The final step of PG biosynthesis in Mtb is catalyzed by two different classes of enzymes, namely the D,D-transpeptidases (also known as Penicillin Binding Proteins – PBPs) and L,D-transpeptidases (Ldts). Conversely, Ldts catalyze the crosslinking of disaccharyl-tetrapeptide polymers by forming a transpeptide bond between the third amino acid in adjacent stem peptides thereby generating 3 → 3 crosslinkages between mDAP residues. Approximately two-thirds of the linkages in Mtb PG are of 3 → 3 type and their synthesis is catalyzed by the Ldts, highlighting the importance of these non-classical transpeptidases to this pathogen. Mtb lacking LdtMt2 is severely attenuated for growth, virulence, has deformed cell walls and exhibits an increased susceptibility to β-lactams.

apo and enzyme reacted with biapenem or tebipenem, and collected X-ray diffraction data at 2.49, 2.18 and 2.45 Å resolutions, respectively. All crystal forms belong to the monoclinic P21 space group with similar cell dimensions and contain two molecules per asymmetric unit. The apo and holo structures show negligible differences among them. The RMSDs are 0.4 and 0.3 Å between apo-LdtMt2 and LdtMt2-biapenem or LdtMt2-tebipenem, respectively, and 0.17 Å between the holo structures for the same 702 aligned Cα atoms aligned. Interestingly, the electron densities in these complexes are similar in size and shape. The observed densities are larger than the glycerol molecule observed in the apo-LdtMt2 crystal form but smaller than expected for an intact biapenem or tebipenem adduct as illustrated in Fig. 1d. The glycerol molecule found in the apo-LdtMt2 crystal form is disconnected at 2.7 Å from the catalytic cysteine and poorly overlapping with the larger and connected MTOA adduct.

>DLLVPKLTASVTDGAVGVTVDAPVSVTAADGVLAAVTMVNENGRPVAGRLSPDGLRWSTTEQLGYNRRYTLNATALGLGGAATRQLTFQTSSPAHLTMPYVMPGDGEVVGVGEPVAIRFDENIADRGAAEKAIKITTNPPVEGAFYWLNNREVRWRPEHFWKPGTAVDVAVNTYGVDLGEGMFGEDNVQTHFTIGDEVIATADDNTKILTVRVNGEVVKSMPTSMGKDSTPTANGIYIVGSRYKHIIMDSSTYGVPVNSPNGYRTDVDWATQISYSGVFVHSAPWSVGAQGHTNTSHGCLNVSPSNAQWFYDHVKRGDIVEVVNTVGGTLPGIDGLGDWNIPWDQWRAGNAK[2x]> MLSIDEAFRKFKSRLELNEREQKNASQRQNEVRDYLQTKFGIARSFLTGSYARYTKTKPLKDIDIFFVLKDSEKHYHGKAASVVLDDFHSALVEKYGSAAVRKQARSINVDFGVHIDAEDNTDYRVVSVDAVPAFDTGDQYEIPDTASGKWIKTDPEIHKDKATAAHQAYANEWKGLVRMVKYWNNNPKHGDLKPVKPSFLIEVMALECLYGGWGGSFDREIQSFFATLADRVHDEWPDPAGLGPAISNDMDAARKQRAQQLLFQASQDASIAIDHARRGRNIEALRAWRALFGPKFPLS;> MSTVATYSYTHSVTYVTDNILKSLKDIILLSGLDPEHFADRWESNTRAIKTWLGTGDLRKVILEI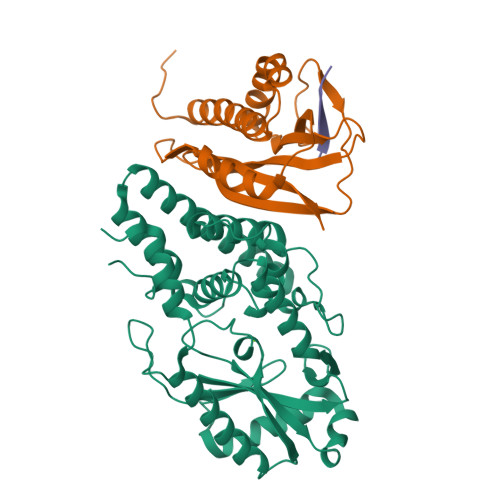YNPATDKLVTRWDIDIVYGWSDGDGSFWTDTEQLKYAIKKAGLLPSQAKYKLMLDTKPGRPDVEGWSKGSYRSTDGMVKQSLGSTVEHSGLAGQAGYWRQR;> SNAEVMEFNP(7R)-6-formyl-7-(4H-pyrazolo[1,5-c][1,3]thiazol-2-yl)-4,7-dihydro-1,4-thiazepine-3-carboxylic acid | C12 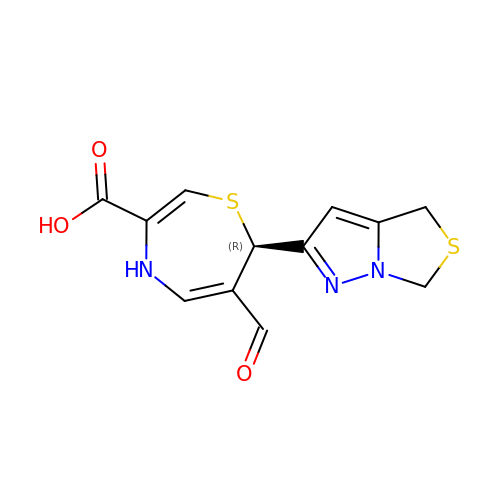H11 N3 O3 S2 | BBUNPRSRYKGFTQ-LLVKDONJSA-N1-[PYRROL-1-YL-2,5-DIONE-METHOXYMETHYL]-PYRROLE-2,5-DIONE | C10 H8 N2 O5 | 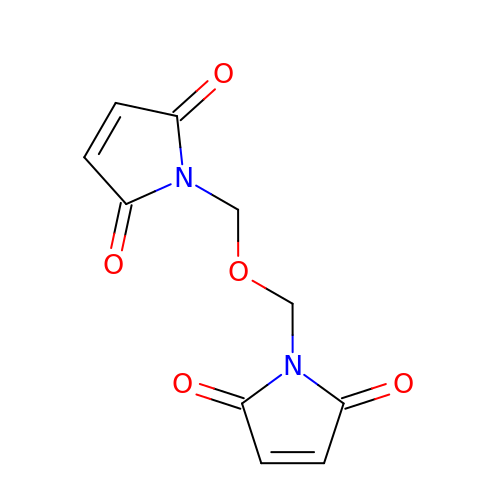UTRLJOWPWILGSB-UHFFFAOYSA-N> MGDCDIEGKDGKQYESVLMVSIDQL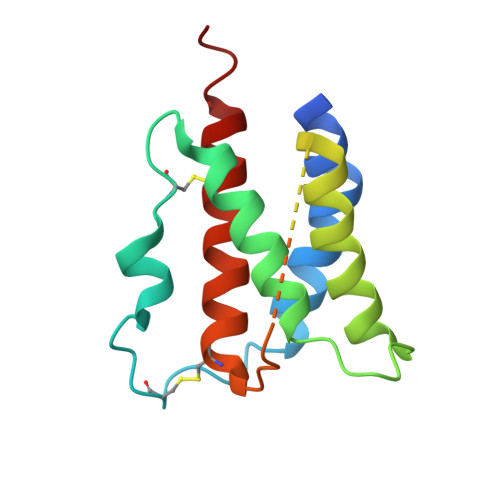LDSMKEIGSNCLNNEFNFFKRHICDANKEGMFLFRAARKLRQFLKMNSTGDFDLHLLKVSEGTTILLNCTGQVKGRKPAALGAAQPTKSLEENKSLKEQKKLNDLCFLKRLLQEIKTCWNKILMGTKEH> GPLGSMSTKTNIQKDW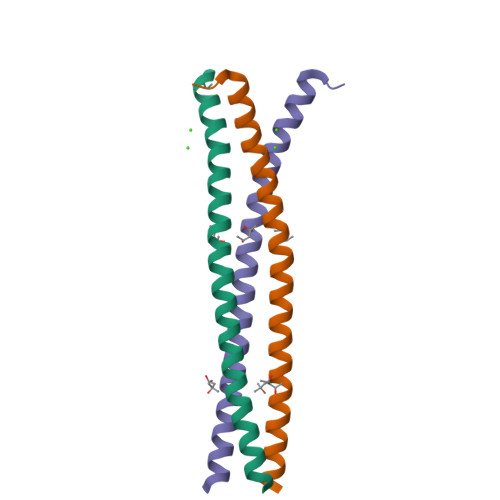EQREFIEDMSINIQKIVEFLNKFELSTRNKLSDLNEKLTILDRQVDYLEATFKTVQE>[2x]MSVEKIPGYTYGETENRAPFNLEDLKLLKEAVMFTAEDEEYIQKAGEVLEDQVEEILDTWYGFVGSHPHLLYYFTSPDGTPNEKYLAAVRKRFSR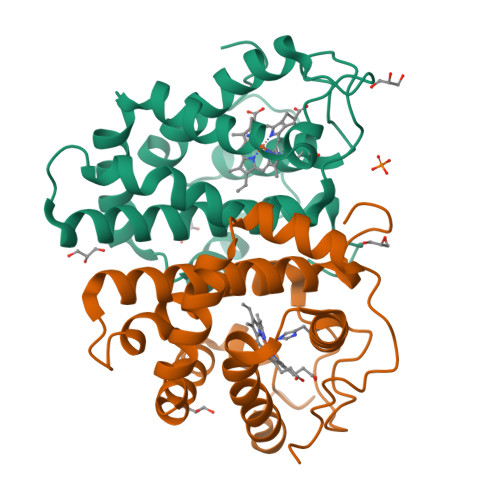WILDTSNRSYDQAWLDYQYEIGLRHHRTKKNQTDNVESVPNIGYRYLVAFIYPITATMKPFLARKGHTPEEVEKMYQAWFKATTLQVALWSYPYVKYGDF>[2x]MAHHHHHHMAASANGSTKGSETDLPIGKDGTTLHLKCKSDELADRIIFVGDPGRVDVISGYFDKDSIRASRDHREIRFATGTYKGTPVTVISTGMGVDNIEIVLNEIHALKEYDMERGQWRHRKGDADAPSAGPFFDPSTMKIIRLGTCGSPAESVPPLALAVTRHAIG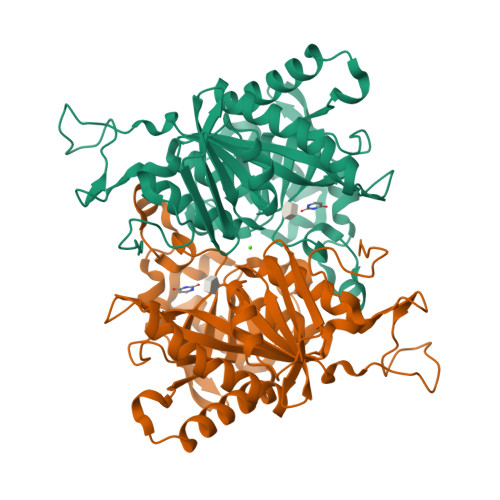MDNTSLYYSAGTRETSKDQQEIRRIVREQTGLRAIDIYTSMAHPNITKSICAACDAHNAATGSEADKQQYVIGTTATASGFYGCQGRRVGRFMKHLTVPNMVEELGSLKFNLSNGVEVVTNIEMETSAICYLSDMLGYQAGAACVVVSKRVGEKKMFLGDQLDAAMKRCIKIILEALVSA>[4x]MEQRASLDSEESESPPQENSCLDPPDRDPNCKPPPVKPHIFTTRSRTRLFGKGDSEEASPLDCPYEEGGLASCPIITVSSVLTIQRPGDGPASVRPSSQDSVSAGEKPPRLYDRRSIFDAVAQSNCQELESLLPFLQRSKKRLTDSEFKDPETGKTCLLKAMLNLHNGQNDTIALLLDVARKTDSLKQFVNASYTDSYYKGQTALHIAIERRNMTLVTLLVENGADVQAAANGDFFKKTKGRPGFYFGELPLSLAACTNQLAIVKFLLQNSWQPADISARDSVGNTVLHALVEVADNTVDNTKFVTSMYNEILILGAKLHPTLKLEEITNRKGLTPLALAASSGKIGVLAYILQREIHEPECRHLSRKFTEWAYGPVHSSLYDLSCIDTCEKNSVLEVIAYSSSETPNRHDMLLVEPLNRLLQDKWDRFVKRIFYFNFFVYCLYMIIFTAAAYYRPVEGLPPYKLKNTVGDYFRVTGEILSVSGGVYFFFRGIQYFLQRRPSLKSLFVDSYSEILFFVQSLFMLVSVVLYFSQRKEYVASMVFSLAMGWTNMLYYTRGFQQMGIYAVMIEKMILRDLCRFMFVYLVFLFGFSTAVVTLIEDGKNNSLPMESTPHKCRGSACKPGNSYNSLYSTCLELFKFTIGMGDLEFTENYDFKAVFIILLLAYVILTYILLLNMLIALMGETVNKIAQESKNIWKLQRAITILDTEKSFLKCMRKAFRSGKLLQVGFTPDGKDDYRWCFRVDEVNWTTWNTNVGIINEDPGNCEGVKRTLSFSLRSGRVSGRNWKNFALVPLLRDASTRDRHATQQEEVQLKHYTGSLKPEDAEVFKDSMVPGEKENSLEVLFQGPDYKDDDDKAHHHHHHHHHH

To address this question, we chose to study transient receptor vanilloid member 1 (TRPV1), which is the receptor for vanilloids and noxious heat. TRPV1 is a homotetramer, where each protomer has an N-terminal cytosolic ankyrin repeat domain (ARD) and a transmembrane domain (TMD) of six transmembrane helices (S1-S6). The TMD is composed of a voltage sensor-like S1-S4 domain (VSLD), a pore domain (S5, the turret, the pore helix (PH), the selectivity filter (SF), the pore loop (PL), and S6), and the amphipathic TRP helix. Vanilloid binding at the S1-S4 domain allosterically acts upon the pore domain, driving pore opening.

Various strategies of 3D classification of the 4 °C dataset consistently resulted in three distinct classes with nearly equal particle distributions to overall excellent quality. For the three classes of RTx-TRPV1 at 4 °C, we assigned class I, class II, and class III according to the size of the pore opening (class I being the narrowest). Based on this criterion, the 4 °C class I represents a nonconducting, closed state whereas class III represents a conducting, open state. Comparing the RTx-bound closed state of TRPV1 (TRPV1C,RTx) with the published apo TRPV1 structure shows that RTx binding induces slight local changes near the vanilloid binding site of the S1-S4 domain (S3, S4b, the S4-S5 linker), but otherwise the conformation remains similar to the apo TRPV1 structure. Because the backbone carbonyl groups of G643 in the SF can coordinate dehydrated Na+, as evidenced by the cryo-EM density maps of the TRPV1C,RTx and the published apo TRPV1, the only residue that can potentially block ion permeation at the SF is M644. In the closed state T641 (PH) and Y584 (S5) interact with each other, but they do not interact with Y666 (S6) which is concomitant with the first S6 dilation. 1 Initially, RTx binds with no significant conformational changes.>[2x]MGTFIQAVDGTKIYVEDIGSGQPVVMLHGWPANNNMFEYQKNRLLEEGYRYIGVDYRGYGKSDAPATGYDYTTMASDINEVIQQLKLTNVT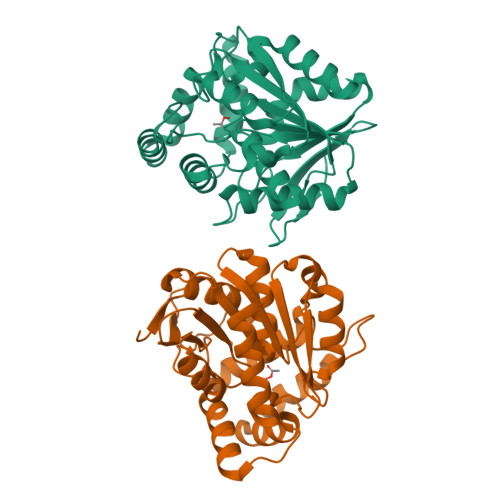LLGFSMGGGIALKYLLNHGESNVSKLILAGAAAPVFTQRDGYPYGMTKDEVDALIEDTKQDRPSMLKGFGEIFFAKEHPEPLQQWFHNLSVDASSHGTIQSAIALRDEDLRDGLPKITVDTLIMHGKKDQVCPFEFAEVMHENIAGSRLEVFEESGHGMFLDEREKFTETLVSYVKSSQTV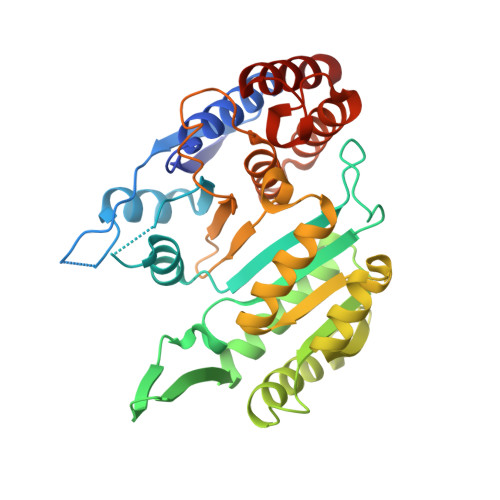> MGSTGGVQTVTLIPGDGIGPEISAAVMKIFDAAKAPIQWEERNVTAIQGPGGKWMIPSEAKESMDKNKMGLKGPLKTPIAAGHPSMNLLLRKTFDLYANVRPCVSIEGYKTPYTDVNIVTIRENTEGEYSGIEHVIVDGVVQSIKLITEGASKRIAEFAFEYARNNHRSNVTAVHKANIMRMSDGLFLQKCREVAESCKDIKFNEMYLDTVCLNMVQDPSQFDVLVMPNLYGDILSDLCAGLIGGLGVTPSGNIGANGVAIFESVHGTAPDIAGKDMANPTALLLSAVMMLRHMGLFDHAARIEAACFATIKDGKSLTKDLGGNAKCSDFTEEICRRVKDLD>[2x]GSHMPESVIQNYNKALQQLEKYKPYEEALLQAEAPRLAEYQAYIDFEMKIGDPARIQLIFERALVENCLVPDLWIRYSQYLDRQLKVKDLVLSVHNRAIRNCPWTVALWSRYLLAMERHGVDHQVISVTFEKALNAGFIQATDYVEIWQAYLDYLRRRVDFKQDSSKELEELRAAFTRALEYLKQEVEERFNESGDPSCVIMQNWARIEARLCNNMQKARELWDSIMTRGNAKYANMWLEYYNLERAHGDTQHCRKALHRAVQCTSDYPEHVCEVLLTMERTEGSLEDWDIAVQKTETRLARVNEQRMKAAEKEAALVQQEEEKAEQRKRARAEKKAL;>GSHMAEGGGCRERPDAETQKSELGPLMRTT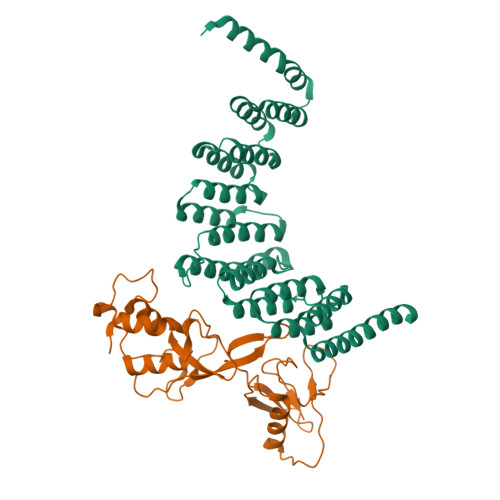LQRGAQWYLIDSRWFKQWKKYVGFDSWDMYNVGEHNLFPGPIDNSGLFSDPESQTLKEHLIDELDYVLVPTEAWNKLLNWYGCVEGQQPIVRKVVEHGLFVKHCKVEVYLLELKLCENSDPTNVLSCHFSKADTIATIEKEMRKLFNIPAERETRLWNKYMSNTYEQLSKLDNTVQDAGLYQGQVLVIEPQNEDGTWPRQTLQ[2x]> GPHMPKGELGAGTPHEPYNLPLRGNPNKSGCHHCLADQCHCVFFERLLDATFRRLDIKRITEVSGSRHLCAKSLLPTFVSRMVRLMEITSEDTFYDLGCGNGSILFQVAFLTGARCVGIEISEHNAKVAKKAWEVIRPELEGSSGRSMSEVNIITSDMTKILADERLFESERGKTVILLSNLLFPKSLTHYLSERFRRVPSGTRILCFDDLYPHSRSVAAIRDPEAFRLFAMTDYRWQECSVEWCTRDGPFFIHRRR

In higher eukaryotes, a single DOT1 histone H3 lysine 79 (H3K79) methyltransferase processively produces H3K79me2/me3 through histone H2B mono-ubiquitin interaction, while the kinetoplastid Trypanosoma brucei di-methyltransferase DOT1A and tri-methyltransferase DOT1B efficiently methylate the homologous H3K76 without H2B mono-ubiquitination. DOT1 enzymes are highly conserved across metazoans and fungi, but not in the early-branched eukaryotic class of kinetoplastids including Trypanosoma brucei subsp., Trypanosoma cruzi, and Leishmania spp. In kinetoplastids, three DOT1-like methyltransferases have been identified, two of which (T. brucei DOT1A and DOT1B) have demonstrated methyltransferase activity toward H3K76 (corresponding to H3K79 in human and yeast) in vivo and in vitro. Both DOT1A and DOT1B represent minimal enzymes with less than 300 residues, comprised of a significantly diverged N-terminal domain (magenta in Fig. 1a, b) and a conserved C-terminal methyltransferase core domain (dark blue) that contains canonical and non-canonical methyltransferase motifs. Based on structural and biochemical analyses of DOT1A, we identify key residues in the methyltransferase motifs VI and X for efficient ubiquitin-independent H3K76 methylation in kinetoplastids. Substitution of a basic to an acidic residue within motif VI (Gx6K) is essential to stabilize the DOT1A enzyme-substrate complex, while substitution of the motif X sequence VYGE by CAKS renders a rigid active-site loop flexible, implying a distinct mechanism of substrate recognition.

To investigate the implications of these differences on the structural level, we determined the X-ray crystal structure of DOT1A and compared it to human and yeast active-form DOT1-nucleosome complexes. Δ42-DOT1A crystallized in complex with the methyl donor product AdoHcy in two different crystal forms (space groups C2221 and P212121), and their structures were determined at 2.1 and 1.9 Å resolution, respectively. The asymmetric units of the C2221 and P212121 space groups contain one and two DOT1A enzymes referred to as Molecules I to III, respectively. All three molecules are highly similar with a root-mean-square deviation (rmsd) of ~0.3 Å comparing 234 pairs of Cα atoms. Hence, we will describe the structure of Molecule I in the C2221 space group and only discuss significant discrepancies among the three molecules. The DOT1A N-terminal domain folds into a Zn-coordinating β-hairpin structure comprising residues Glu46 to Cys79. The β-hairpin structure is tightly associated with the methyltransferase core domain through a hydrogen bond network by extending the antiparallel β-sheet of the methyltransferase core domain. Therefore, the N-terminal β-hairpin structure appears to stabilize the DOT1A methyltransferase core domain.> MLKAWHLPVAPFIKEQQERLMITLWLSGDDLPPRVTLRAEEDNEELSLPMHRLRQAPHPGVVAWRGEINLVNGQPRRRYSFKLLWADRQLWFTPQEFNRFPPARLEQFAVDLPDSGPQWVADQVFYQIFPDRFARSQSREAEQDATYYHHAAGHDIVRKAWDEPLTAEAGGSTFYGGDLDGISEKLPYLKQLGVTALYLNPVFVAPSVHKYDTEDYRRVDPQFGGDAALLRLRHNTQKEGMRLILDGVFNHSGDSHAWFDRHQRGSGGACHNADSPWRDWYNFSPEGVAHDWLGYASLPKLDYRSSTLIDEIYGGEDSVVRHWLKAPWSMDGWRLDVVHMLGEGGGARNNLRHIAGITQAAKLERPDAFV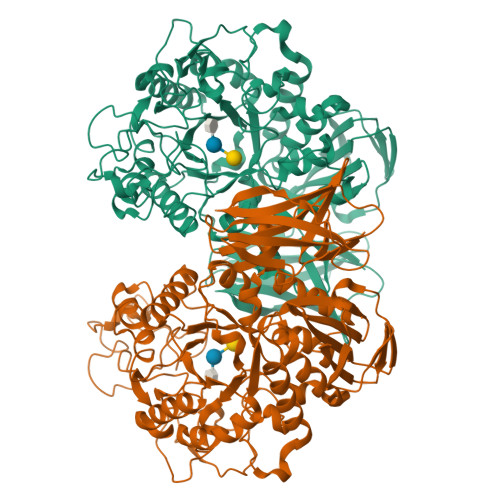FGEHFGDARQWLQADVEDSAMNYRGFTFPLWGFLANTDISYDPQKIDAQTCMAWMDNYRAGLSHQQQLRMFNQLDSHNTARFKSLLGKDVARLPLAVVWLFSWPGVPCIYYGDEVGVDGNNDPFCRKPFPWDPALQDGDLLDLYKRMSKLRKAHQALRYGGCQVIYAEDNVVVFVRVYKQQRVLVAINRGEACEVVIEDSPLLDVNGWQLKEGAGALHDGVLTLPAISASVWFSR>GSMAVTNVAELNALVERVKKAQREYASFTQEQVDKIFRAAALAAADARIPLAKMAVAESGMGIVEDKVIKNHFASEYIYNAYKDEKTCGVLSEDDTFGTITIAEPIGIICGIVPTTNPTSTAIFKSLISLKTRNAIIFSPHPRAKDATNKAADIVLQAAIAAGAPKDLIGWIDQPSVELSNALMHHPDINLILATGGPGMVKAAYSSGKPAIGVGAGNTPVVIDETADIKRAVASVLMSKTFDNGVICASEQSVVVVDSVYDAVRERFATHGGYLLQGKELKAVQDVILKNGALNAAIVGQPAYKIAELAGFSVPENTKILIGEVTVVDESEPFAHEKLSPTLAMYRAKDFEDAVEKAEKLVAMGGIGHTSCLYTDQDNQPARVSYFGQKMKTARILINTPASQGGIGDLYNFKLAPSLTLGCGSWGGNSISENVGPKHLINKKTVAKRAENMLWHKLPKSIYFRRGSLPIALDEVITDGHKRALIVTDRFLFNNGYADQITSVLKAAGVETEVFFEVEADPTLSIVRKGAELANSFKPDVIIALGGGSPMDAAKIMWVMYEHPETHFEELALRFMDIRKRIYKFPKMGVKAKMIAVTTTSGTGSEVTPFAVVTDDATGQKYPLADYALTPDMAIVDANLVMDMPKSLCAFGGLDAVTHAMEAYVSVLASEFSDGQALQALKLLKEYLPASYHEGSKNPVARERVHSAATIAGIAFANAFLGVCHSMAHKLGSQFHIPHGLANALLICNVIRYNANDNPTKQTAFSQYDRPQARRRYAEIADHLGLSAPGDRTAAKIEKLLAWLETLKAELGIPKSIREAGVQEADFLANVDKLSEDAFDDQCTGANPRYPLISELKQILLDTYYGRDYVEGETAAKKEAAPAKAEKKAKKSA[6x]

Aldehyde–alcohol dehydrogenase (AdhE) is a multifunctional enzyme containing two enzymatic domains responsible for aldehyde dehydrogenase (ALDH) and alcohol dehydrogenase (ADH) activities. AdhE is a bifunctional enzyme having two catalytic activities responsible for two consecutive reactions converting acetyl-CoA to ethanol. AdhE forms long helical filaments called spirosome and this spirosome formation is critical for the AdhE activity. In addition, AdhE spirosomes undergo a structural transition from a compact to an extended form, in the presence of cofactors.

Here, we present the atomic resolution (3.43 Å) cryo-EM structure of AdhE in an extended spirosome form in the presence of cofactors. We found that AdhE stably exists as an extended spirosome form in the presence of Zn2+, NAD+, and ethanol. The cryo-EM structure reveals that AdhE forms a right-handed spirosome with 130 Å width, and four AdhE molecules make one helical turn with a pitch of 120 Å, which is consistent with the previous SAXS analysis on an extended AdhE spirosome. In one helical turn, ALDH and ADH domains from two AdhE molecules are intertwined to form a dimer, and two dimers make a tetramer by interacting with each other via their ADH domains. In the cryo-EM structure, there are clear densities of NAD+ in both the ALDH and ADH domains, and Zn2+ in the ADH domain. The AdhE dimer in an extended spirosome is widened by about 10° compared with the dimer in the compact spirosome. In contrast, in the extended conformation where NAD+ is bound, the NAD+ binding pocket is widely exposed. In the extended AdhE spirosome, both the ALDH and ADH catalytic sites are readily accessible to solvent from the outside as well as the inside of the spirosome. Furthermore, the interaction between the ALDH and ADH domains of two different AdhE molecules creates a channel between the two catalytic sites, which is located at the inside of the spirosome. Considering that ALDH and ADH catalytic activities mediate consecutive reactions converting acetyl-CoA to ethanol via acetaldehyde as an intermediate, it is likely that the channel observed plays a role in conveying the intermediate product.>SHRNEAGHGDLHEILHEAVPLDANEREILELKEDAFAQRRREIETRLRAANGKLADAIAKNPAWSPEVEAATQE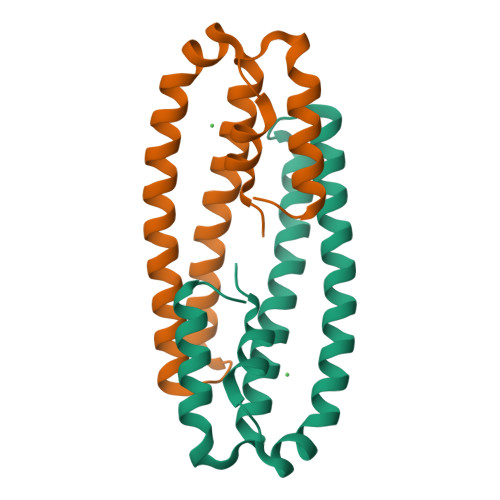VERAAGDLQRATLVHVFECRAGLKPEHRPAYDRVLIDALRRGSQ[2x]> ARTVVLITGCSSGIGLHLAVRLASDPSQSFKVYATLRDLKTQGRLWEAARALACPPGSLETLQLDVRDSKSVAAARERVTEGRVDVLVCNAGLGLLGPLEALGEDAVASVLDVNVVGTVRMLQAFLPDMKRRGSGRVLVTGSVGGLMGLPFNDVYCASKFALE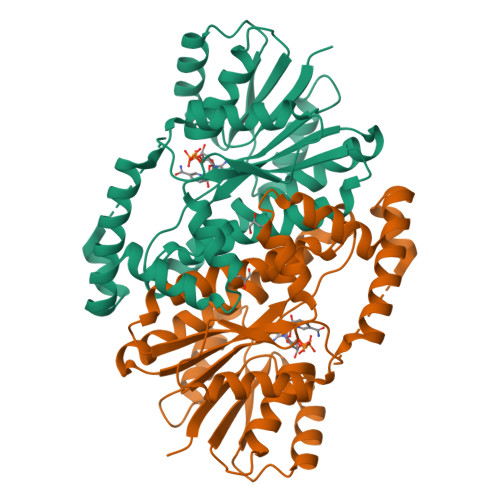GLCESLAVLLLPFGVHLSLIECGPVHTAFMEKVLGSPEEVLDRTDIHTFHRFYQYLAHSKQVFREAAQNPEEVAEVFLTALRAPKPTLRYFTTERFLPLLRMRLDDPSGSNYVTAMHREVFGDVPAKAEAGAEAGGGAGPGAEDEAGRSAVGDPELGDPPAAPQ The PotD-PotABC protein complex in Escherichia coli, belonging to the adenosine triphosphate–binding cassette transporter family, is a spermidine-preferential uptake system. In general, ATP binding, hydrolysis, and phosphate release trigger conformational changes in the transporter, leading to the uptake of extracellular polyamines. Here, we report structural details of the polyamine uptake system PotD-PotABC in various states.

Thus, the PotD-PotABC complex was formed by incubating the purified PotD protein with the PotABC E173Q complex in the presence of Spd, ATP, and Mg2+. The architecture of the entire PotD-PotABC complex reveals an inward-facing conformation, assigned as the pretranslocation state. Notably, only two pairs of hydrogen bonds are formed between the PotD N-lobe and PotB, namely, the main chain oxygen atom of Y56 and the hydroxyl group of T58 in PotD interact with the amine group of K217 and the hydroxyl group of S220 in PotB, respectively. In contrast, the interaction between the PotD C-lobe and PotBC is more extensive. Namely, the residues D212 to E222 in PotD are sandwiched between PotC and PotB, establishing extensive contacts. In particular, the residues E220 to E222 in PotD interact with the residues K127, T126, and R145 in PotC through three pairs of hydrogen bonds. We observed one Spd molecule bound inside the PotD. In the pretranslocation state, Spd is enclosed by the N- and C-lobes of PotD in a tightly “closed” form. The Spd-bound PotD in a closed form interacts with the PotABC complex to form the entire PotD-PotABC complex in the pretranslocation state (state 2).

>[2x]MGQSKKLNKQPSSLSPLVQLAGIRKCFDGKEVIPQLDLTINNGEFLTLLGPSGCGKTTVLRLIAGLETVDSGRIMLDNEDITHVPAENRYVNTVFQSYALFPHMTVFENVAFGLRMQKTPAAEITPRVMEALRMVQLETFAQRKPHQLSGGQQQRVAIARAVVNKPRLLLLDQSLSALDYKLRKQMQNELKALQRKLGITFVFVTHDQEEALTMSDRIVVMRDGRIEQDGTPREIYEEPKNLFVAGFIGEINMFNATVIERLDEQRVRANVEGRECNIYVNFAVEPGQKLHVLLRPEDLRVEEINDDNHAEGLIGYVRERNYKGMTLESVVELENGKMVMVSEFFNEDDPDFDHSLDQKMAINWVESWEVVLADEEHK;> MKNTSKFQNVVIVTIVGWLVLFVFLPNLMIIGTSFLTRDDASFVKMVFTLDNYTRLLDPLYFEVLLHSLNMALIATLACLVLGYPFAWFLAKLPHKVRPLLLFLLIVPFWTNSLIRIYGLKIFLSTKGYLNEFLLWLGVIDTPIRIMFTPSAVIIGLVYILLPFMVMPLYSSIEKLDKPLLEAARDLGASKLQTFIRIIIPLTMPGIIAGCLLVMLPAMGLFYVSDLMGGAKNLLIGNVIKVQFLNIRDWPFGAATSITLTIVMGLMLLVYWRASRLLNKKVELE;> MIGRLLRGGFMTAIYAYLYIPIIILIVNSFNSSRFGINWQGFTTKWYSLLMNNDSLLQAAQHSLTMAVFSATFATLIGSLTAVALYRYRFRGKPFVSGMLFVVMMSPDIVMAISLLVLFMLLGIQLGFWSLLFSHITFCLPFVVVTVYSRLKGFDVRMLEAAKDLGASEFTILRKIILPLAMPAVAAGWVLSFTLSMDDVVVSSFVTGPSYEILPLKIYSMVKVGVSPEVNALATILLVLSLVMVIASQLIARDKTKGNTGDVK;> MKKWSRHLLAAGALALGMSAAHADDNNTLYFYNWTEYVPPGLLEQFTKETGIKVIYSTYESNETMYAKLKTYKDGAYDLVVPSTYYVDKMRKEGMIQKIDKSKLTNFSNLDPDMLNKPFDPNNDYSIPYIWGATAIGVNGDAVDPKSVTSWADLWKPEYKGSLLLTDDAREVFQMALRKLGYSGNTTDPKEIEAAYNELKKLMPNVAAFNSDNPANPYMEGEVNLGMIWNGSAFVARQAGTPIDVVWPKEGGIFWMDSLAIPANAKNKEGALKLINFLLRPDVAKQVAETIGYPTPNLAARKLLSPEVANDKTLYPDAETIKNGEWQNDVGAASSIYEEYYQKLKAGR>[2x]MYGAGQIQVLEGLEAVRKRPGMYIGSTSERGLHHLVWEIVDNS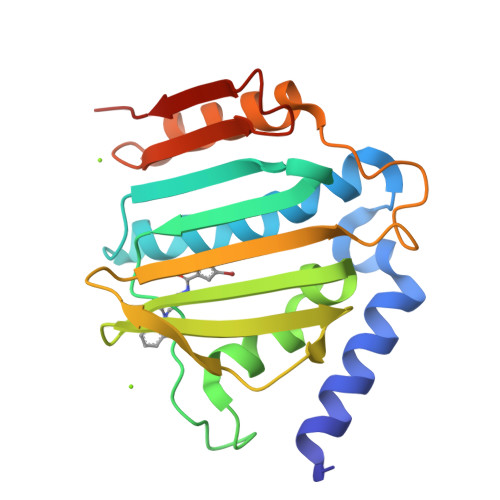IDEALAGYANQIEVVIEKDNWIKVTDNGRGIPVDIQEKMGRPAVEVILTSSVVNALSQDLEVYVHRNETIYHQAYKKGVPQFDLKEVGTTDKTGTVIRFKADGEIFTETTVYNYETLQQRIRELAFLNKGIQITLRDERDEENVREDSYHYEGGI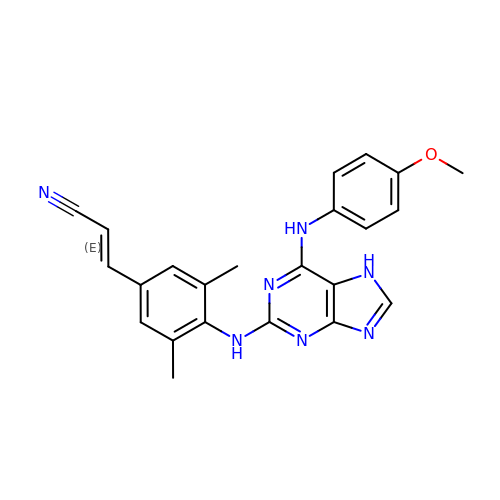(2E)-3-[4-({6-[(4-methoxyphenyl)amino]-7H-purin-2-yl}amino)-3,5-dimethylphenyl]prop-2-enenitrile | C23 H21 N7 O | IDEUQSZAIWGGSN-SNAWJCMRSA-N We discover FucOB from the mucin-degrading bacteria Akkermansia muciniphila as an α-1,2-fucosidase able to hydrolyze Type I, Type II, Type III and Type V H antigens to obtain the afucosylated Bombay phenotype in vitro. FucOB displays α-1,2-L-fucosidase activity and showed no activity against α-1,3, α-1,4, and α-1,6 fucosylated oligosaccharides. A close inspection of the crystal structure revealed that FucOB crystallized as a monomer comprising three domains from the N- to the C-terminus: (i) a β-sandwich domain (residues 25–260), (ii) an (α/α)6 helical barrel catalytic domain (residues 357–712) and (iii) a second β-sandwich domain (residues 713–785). FucOB as well as other members of the GH95 family follow a single displacement inverting catalytic mechanism.

A conserved glutamic acid (E541 in FucOB) acts as a general acid catalyst. Mutation of E541 by alanine completely abolished the hydrolytic activity of the enzyme (see below). To further understand the FucOB substrate specificity at the molecular level, we performed co-crystallization experiments with (i) wild-type FucOB and (ii) the catalytically inactive variant FucOBE541A, both in the presence of V Type H blood group antigen as the substrate. Despite many efforts, we could not crystallize FucOB or FucOBE541A in the presence of the substrate or the corresponding product. The structural comparison of FucOB and the FucOBE541A revealed that the protein structure is mostly preserved and that there are no substantial conformational changes (r.m.s.d. of 0.477 Å for 761 residues). The crystal packing analysis of FucOB and FucOBE541A structures reveals a strong π–π stacking interaction between W453 with two prolines residues, P765 and P783, of the neighbor protomer. Consequently, this protomer restricts the entrance of the substrate into the active site, supporting the inability to obtain a complex crystal form. To determine whether FucOB can convert universal O into a rare Bombay type blood group, type O RBCs were incubated with 200, 50, 5, 0.5, 0.05, and 0.005 µg mL−1 of either FucOB or the catalytically inactive version of the enzyme FucOBE541A, and analyzed by agglutination assays against naturally containing anti-H Bombay serum (see the “Methods” section). In contrast, the catalytically inactive FucOBE541A showed a clear agglutination reaction after treatment with the anti-H lectin.

> MHHHHHHENLYFQGSGADKPSASNLIWSDEPAVVVYPQEDKNSEGSFGKYRKPASVWEAEGYPIGNGRVGAMIFSAPGRERLALNEISLWSGGANPGGGYGYGPDAGTNQFGNYLPFGDLFVDFKKGDQPASLSVEDFTRSLDLRDGIHKVNYKADGVTYDREAFSSTPANVLVLNYKASKPGQFSADFSVNSQLGADISAKGSVITWKGMLKNGMNYEGRVLIRPKGGTLSASGDKISVKNADSCMVVIAMETDYLMDYKKDWKGESPSRKLDRYAAKAASADYAALKQAHISQYKSMFDRVKVNFGKTEEDVAKLPTPKRLEAYKKNPADPDLEETMFQFGRYLLLSSSRPGTLPANLQGLWNDYVKPPWACDYHNNINVQMAYWGAEPANLSECHEALVNYVEAMAPGCRDASQANKGFNTKDGKPVRGWTVRTSQNIFGGNGWQWNIPGAAWYALHIWEHYAFTGDRKYLEKQAYPLMKEICHFWEDHLKELGAGGEGFKTNGKDPSEEEKKDLADVKAGTLVAPNGWSPAHGPREDGVMHDQQLIAELFSNTIKAARILGKDAAWAKSLEGKLKRLAGNKIGKEGNLQEWMIDRIPKTDHRHTSHLFAVFPGNQISKLKTPKLAEAARLSLEWRGTTGDSRRSWTWPWRTALWARLGEGNKAHEMVQGLLKFNTLPNMLTTHPPMQMDGNFGIVGGICEMLVQSHAGGLDIMPSPVEAWPEGSVKGLKARGNVTVDFSWKDGKVSNVKLYSAQPKVLPVRVNGKMTRMKTLPLKSGAGSSQPAAR> MKLLTTAILSSAIALSSMAAAAGTDNPTVAKKTVSYVCQQGKKVKVTYGFNKQGLTTYASAVINGKRVQMPVNLDKSDNVETFYGKEGGYVLGTGVMDGKSYRKQPIMITAPDNQIVFKDCSPR

Recently, we described a novel adhesin termed the Adhesin Complex Protein (ACP—NMB2095/NEIS2075), a conserved protein found in the OM of meningococci, gonococci, N. lactamica and all other Neisseria spp.. Nm-ACP acts as a minor adhesin, mediating the adherence of meningococci principally with epithelial cells. In summary, we have identified a new function for Neisseria ACP as an OM-located, surface-exposed lysozyme inhibitor, in addition to its role as an adhesin and as a potential vaccine candidate. ACP is found in all pathogenic and commensal Neisseria spp., and despite structural similarity to the MliC/PliC family proteins, it shares no conserved motifs involved in lysozyme inhibition.

Crystallization trials were initiated on the purified protein, and native data were collected from a single crystal to 1.4 Å resolution. The structure was solved by single wavelength anomalous diffraction from iodide ions, following a soak of a crystal in 0.4 M potassium iodide. The overall fold of Nm-ACPI is close to an 8-stranded β-barrel, stabilized by a disulphide bond between cysteine residues on the first and last β-sheet. However, there are few main-chain hydrogen bonds linking β4-β5 and β8-β1, meaning that the structure divides into two four-stranded anti-parallel β-sheets (β1-β4 and β5-β8). The interaction between β8 and β1 is stabilised by the disulphide bridge between Cys38 and Cys121. The computed surface electrostatic charge distribution showed that the face of the β1-β4 sheet is predominantly basic, whereas the β5-β8 sheet is more apolar, apart from the loop between β4 and β5. All three structures superposed onto Nm-ACPI with r.m.s. deviations of less than 2.0Å, and all preserved the same eight stranded β-fold, although sequence identity with Nm-ACPI was less than 20% in each case. In addition, we noticed that loop 4 from the MliC/PliC family proteins, which occupies the lysozyme active site, corresponded to loop 4 of Nm-ACPI, but was longer in the latter by 3 residues. The sequence motifs SxSGAxY and YxxxTKG, which were conserved in the MliC/PliC family proteins, were not retained in Nm-ACPI. Interestingly, the face associated with the N-terminal region of Neisseria ACP and opposite to the predicted HL-binding site, is highly positively charged, which could provide ACP with the ability to associate with negatively charged surfaces and possibly mediate attachment to the membrane or capsule surface.> PMEFEWDANKAKSNLRKHGVRFED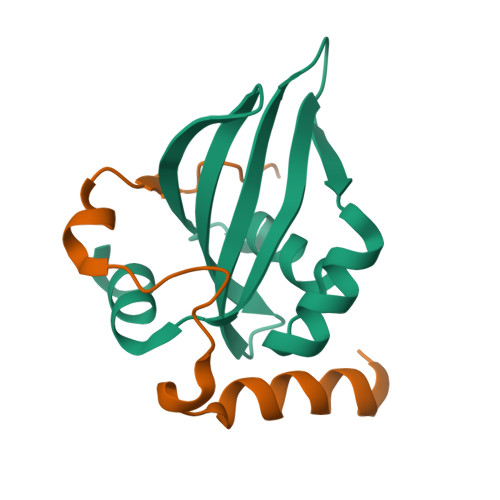AVLVFDDPRHLSRQERYENGEYRWQTLGLVHGIVVILVAHSVRFESGFDVIRIISARKADRKERNRYEHG;> LSAQHEAELKALAKKSDDEIDYSDIPASEDGQWSEAVRGKFFRP> MERYENLFAQLNDRREGAFVPFVTLGDPGIEQSLKIIDTLIDAGADALELGVPFSDPLADGPTIQNANLRAFAAGVTPAQCFEMLALIREKHPTIPIGLLMYANLVFNNGIDAFYARCEQVGVDSVLVADVPVEESAPFRQAALRHNIAPIFICPPNADDDLLRQVASYGRGYTYLLSRSGVTGAENRGALPLHHLIEKLKEYHAAPALQGFGISSPEQVSAAVRAGAAGAISGSAIVKIIEKNLASPKQMLAELRSFVSAMKAASRA;> MTTLLNPYFGEFGGMYVPQILMPALNQLEEAFVSAQKDPEFQAQFADLLKNYAGRPTALTKCQNITAGTRTTLYLKREDLLHGGAHKTNQVLGQA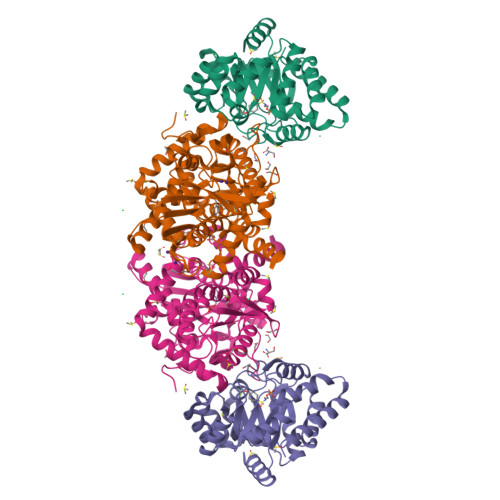LLAKRMGKSEIIAETGAGAHGVASALASALLGLKCRIYMGAKDVERQSPNVFRMRLMGAEVIPVHSGSATLKDACNEALRDWSGSYETAHYMLGTAAGPHPYPTIVREFQRMIGEETKAQILDKEGRLPDAVIACVGGGSNAIGMFADFINDTSVGLIGVEPGGHGIETGEHGAPLKHGRVGIYFGMKAPMMQTADGQIEESYSISAGLDFPSVGPQHAYLNSIGRADYVSITDDEALEAFKTLCRHEGIIPALESSHALAHALKMMREQPEKEQLLVVNLSGRGDKDIFTVHDILKARE> MASARESTPRYLTLIGATLACSALALGAAQAQTEPAEPEAPAETAAADAAGQTEGQRGAAEAAAALAAGEADEPVILEAPAPDARRVYIQDPAHFAAITQQFVIDGSTGRILGMTDGGFLPHPVAAEDGSFFAQASTVFERIARGKRTDYVEVFDPVTFLPIADIELPDAPRFLVGTYQWMNALTPDNKNLLFYQFSPAPAVGVVDLEGKTFDRMLDVPDCYHIFPASPTVFYMNCRDGSLARVDFADGETKVTNTEVFHTEDELLINHPAFSL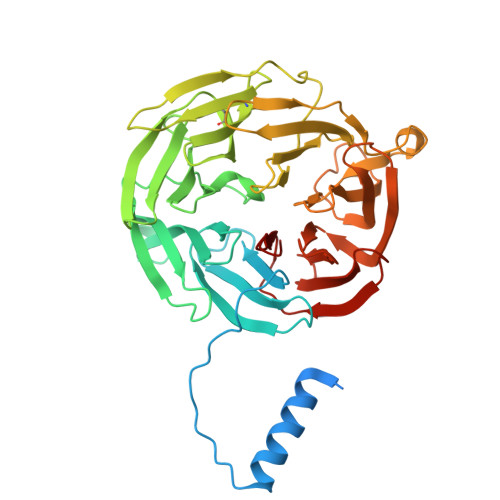RSGRLVWPTYTGKIFQADLTAEGATFRAPIEALTEAERADDWRPGGWQQTAYHRQSDRIYLLVDQRDEWKHKAASRFVVVLNAETGERINKIELGHEIDSINVSQDAEPLLYALSAGTQTLHIYDAATGEELRSVDQLGRGPQIITTHDMDS>MTSAEMTSPNNNSEHQAIAKMRTMIEGFDDISHGGLPIGRSTLVSGTSGTGKTLFSIQFLYNGIIEFDEPGVFVTFEETPQDIIKNARSFGWD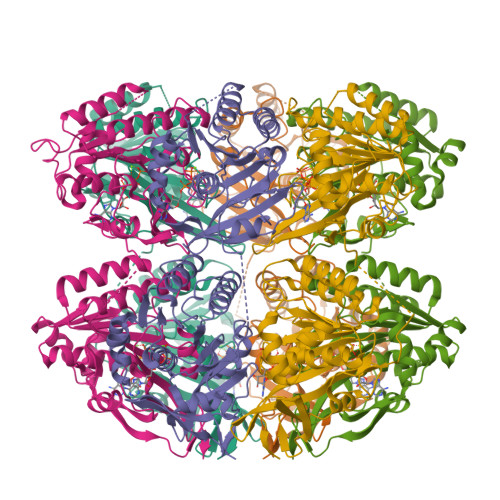LAKLVDEGKLFILDASPDPEGQEVVGGFDLSALIERINYAIQKYRARRVSIDSVTSVFQQYDASSVVRRELFRLVARLKQIGATTVMTTERIEEYGPIARYGVEEFVSDNVVILRNVLEGERRRRTLEILKLRGTSHMKGEYPFTITDHGINIFPLGAMRLTQRSSNVRVSSGVVRLDEMCGGGFFKDSIILATGATGTGKTLLVSRFVENACANKERAILFAYEESRAQLLRNAYSWGMDFEEMERQNLLKIVCAYPESAGLEDHLQIIKSEINDFKPARIAIDSLSALARGVSNNAFRQFVIGVTGYAKQEEITGLFTNTSDQWMGAHSITDSHISTITDTIILLQYVEIRGEMSRAINVFKMRGSWHDKAIREFMISDKGPDIKDSFRNFERIISGSPTRITVDEKSELSRIVRGVQEKGPES[2x]> RNILTNDEGLYAGQSLDVNPYHFIMQEDCNLVLYDHSTSVWASNTGILGKKGCKAVLQADGNFVVYDAEGRSLWASHSVRGNGNYVLVLQEDGNVV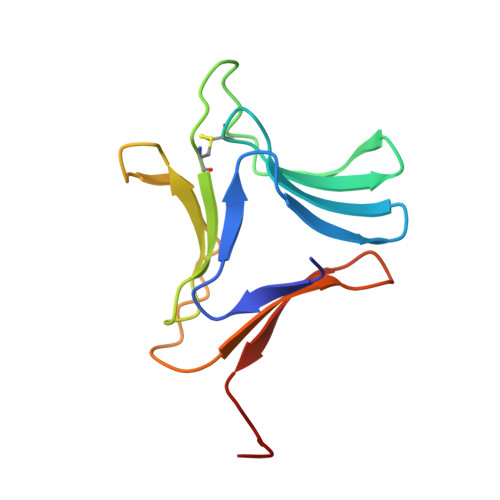IYGSDIWSTN> MSNISRQAYADMFGPTVGDKVRLADTELWIEVEDDLTTYGEEVKFGGGKVIRDGMGQGQMLAADCVDLVLTNALIVDHWGIVKADIGVKDGRIFAIGKAGNPDIQPNVTIPIGA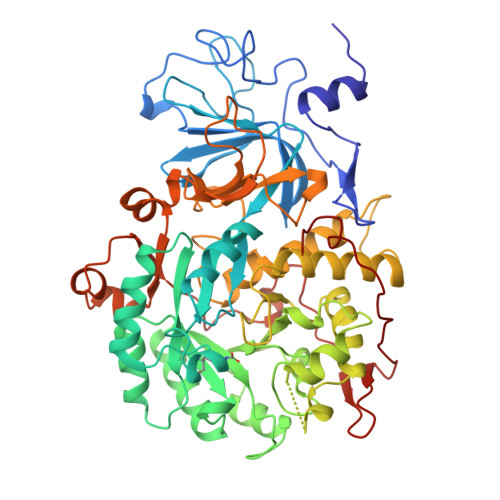ATEVIAAEGKIVTAGGIDTHIHWICPQQAEEALVSGVTTMVGGGTGPAAGTHATTCTPGPWYISRMLQAADSLPVNIGLLGKGNVSQPDALREQVAAGVIGLKIHEDWGATPAAIDCALTVADEMDIQVALHSDTLNESGFVEDTLAAIGGRTIHTFHTEGAGGGHAPDIITACAHPNILPSSTNPTLPYTLNTIDEHLDMLMVDHHLDPDIAEDVAFAESRIRRETIAAEDVLHDLGAFSLTSSDSQAMGRVGEVILRTWQVAHRMKVQRGALAEETGDNDNFRVKRYIAKYTINPALTHGIAHEVGSIEVGKLADLVVWSPAFFGVKPATVIKGGMIAIAPMGDINASIPTPQPVHYRPMFGALGSARHHCRLTFLSQAAAANGVAERLNLRSAIAVVKGCRTVQKADMVHNSLQPNITVDAQTYEVRVDGELITSEPADVLPMAQRYFLF>SFGRDACSEMSIDGLCQCAPIMSEYEIICPANAENPTFRLTIQPKDYVQIMCNLTDTTDYQQLPKKLRIGEVDRVQMRRCMLPGHTPIASILDYLGIVSPTTLIFESDNLGMNITRQHLDRLHGLKRFRFTTRRLTHIPANLLTDMRNLSHLELRANIEEMPSHLFDDLENLESIEFGSNKLRQMPRGIFGKMPKLKQLNLASNQLKSVPDGIFDRLTSLQKIWLHTNPWDCSCPRIDYLSRWLNKNSQKEQGSAKCSGSGKPVRSIICPTTGENLYFQ[2x]

Toll is a transmembrane glycoprotein that functions as a cytokine receptor and is critically involved in both embryonic development and immunity in fruit flies. It is the founding member of an important family of germ-line-encoded pathogen pattern-recognition receptors in mammals, the Toll-like receptors (TLRs). In this study we used the N-terminal domain of Toll encompassing the 201 first amino acids produced as a VLR hybrid protein, a strategy that can generate stable deletion constructs established for mammalian TLRs. Here a counter-diffusion method was used to improve the X-ray diffraction quality of the N-terminal domain of Drosophila melanogaster Toll receptor crystals.

Upon structure determination using a combination of single-wavelength anomalous dispersion of the iodinated species and molecular replacement the atomic structure of the protein could be analysed and the crystal contacts revealed. The atomic structures were determined for both native and derivative forms at 2.4 and 3.0 Å, respectively. The derivative crystals diffracted to a much lower resolution (3.0 Å for the best data set) than the native ones (best at 2.4 Å). According to their respective solvent content of 62 and 59% for the native and derivative crystals, the latter were expected to diffract better. Either incomplete substitution or the additional handling during back-soaking was detrimental to the quality of the derivative crystals. Surprisingly native and derivative crystals were found to belong to different space groups even though they had similar bipyramidal morphologies. However, I3C binding at the concave side of each protein, interacting with charged residues of the leucine-rich repeat region, modifies the packing of the second molecule by tilting it along its long axis by approximately 40° compared to the native structure. This in turn increases the crystal symmetry. The fact that the protein crystallized in two different space groups suggests that the Liesegang-like phenomenon is independent of crystal packing.>NSDNNTDGLIFSPLPQNKNTVVRHYSNEQEMPNLSQMAQRTIDFPTQIVRVSGNLTGLELSCDDVENEIDQVFSKKISPNLFTYNTYVSCGYDVNDPEQHAINFSIQSYFDPLTDNAVDYLKSYLKEYNGYNLFNTTTLQIENAKGIIVSMNLNAGLKSNPDKTPFTLYRQDRNNFYFKSNFDVRKELISDIYQRFYSNDPDMILPFFDKWIFSYAGSVYYSILMASNYLELQPERIFVMENE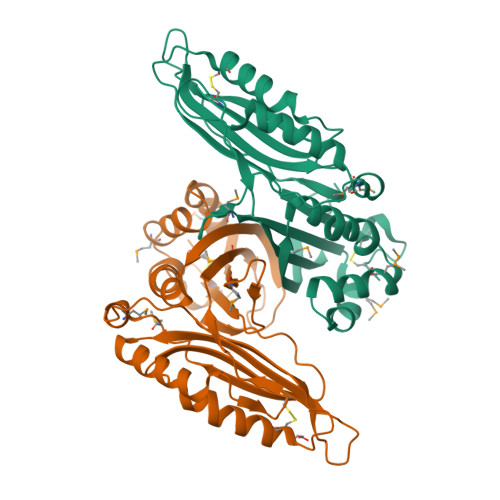GDIFVSDLRYYFANLCMKRNPNKHCL[2x]>[2x]AKPTKVTLVKSAK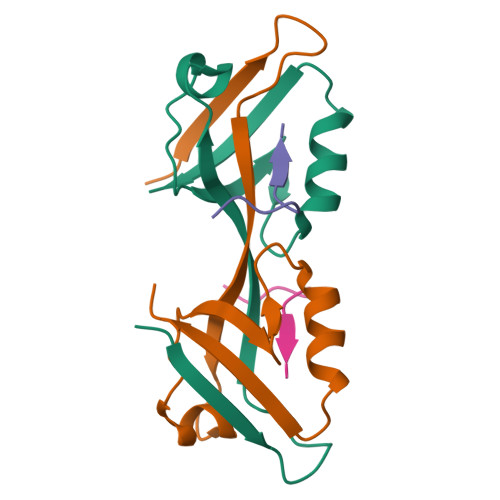NEEYGLRLASHIFVKEISQDSLAARDGNIQEGDVVLKINGTVTENMSLTDAKTLIERSKGKLKMVVQRDERATLLNVPD;>RPRPDDLEI[2x]Depending on the biotinylated metallocofactor, the assembled ArMs exhibit a diverse range of activities. Herein, we report on an artificial nickel chlorinase (ANCase) for the C(sp3)–H chlorination of alkanes, taking advantage of the biotin-Sav technology, Scheme 1c. Sav is a homotetrameric protein with four free biotin-binding sites (four FBS) consisting of two pairs of close-lying bis-biotin binding sites. The pronounced affinity of biotin for Sav ensures the tight binding of a biotinylated metallocofactor to the Sav scaffold.

To maintain the C2-symmetry of the metallocofactor, we set out to attach the biotin anchor to the bridging carbon atom flanked by the two amido-quinoline moieties. Additionally, we converted the original dimethyl group to a cyclohexyl entity to minimize the influence on the dihedral angle between the two amido-quinoline planes. Accordingly, the cofactor [(BiotC4-bAQ)Ni] 1 was synthesized, see, Scheme S1 (ESI†). For this purpose, we assessed the quantitative anchoring of the [(BiotC4-bAQ)Ni] 1 into Sav WT by a HABA displacement titration using CD spectroscopy as readout. The determined dissociation constant was Kd = 0.29 ± 0.05 μM (see ESI†). Upon incorporation into Sav WT, [(BiotC4-bAQ)Ni] 1·Sav WT hereafter, the resulting ArM afforded significantly higher TON (TON = 54), underscoring the positive influence of the second coordination sphere provided by Sav on chlorinase activity. Based on the collected datasets, it is apparent that the [(BiotC4-bAQ)Ni] 1 lies close to residues N49, S112, K121, L124 as well as K121′ from the adjacent monomer. Residue N49 establishes hydrogen bonding interaction with the cyclohexyl amine moiety of the cofactor [(BiotC4-bAQ)Ni] 1. Residues S112 and L124 collectively constitute a hydrophobic pocket, accommodating the cofactor, see Fig. S2 (ESI†). Based on the structural information, we performed genetic optimization of [(BiotC4-bAQ)Ni] 1·Sav WT targeting positions Sav S112 and K121.

>[4x]MASMTGGQQMGRDQAGITGTWYNQLGSTFIVTAGADGALTGTYESAVGNAESRYVLTGRYDSAPATDGSGTALGWTVAWKNNYRNAHSATTWSGQYVGGAEARINTQWLLTSGTTEANAWKSTLVGHDTFTKVKPSAASIDAAKKAGVNNGNPLDAVQQ>[2x]GSHMPAAVSDADFATLEKTSGGRLGVCLWHPASGARYGHRMDERFPMCSTVKFPLAAAILHRVDAGKLSLDQRVAVRQGDIISHSPFTERHVGKDMTVRDLCRATLIIS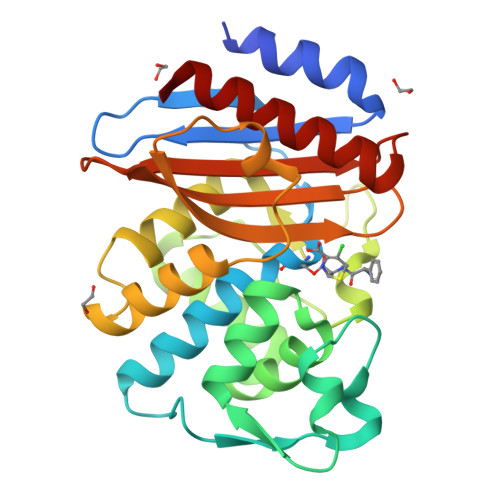DNAAANLLLPLIDGPAGLTAFLQAQGDRITVSARNQPELNHFAPGDPRDTTSPAAMAGNLQRFLLGDVLSPASRQQLADWLIDNQTGDARLRAGLPQGWRVGDKTGSNGQDTSNDIAALWPLAGGAPWLLSCYLQGSALDDDGRDGILRQVGELAGARLG> SSFKKILGLSSKSHKKSKKMGLPPPYDESSPMETQPSAPLSNDFFGMEDMDLYDKDSLRYEKFRFMLKMTVRSNKPFRSYDDVTAAVSQWDNSYIGMVGKRPFYKIIALIGSSHLQATPAVLADLNQPEYYATLTGRCFLPHRLGLIPPMFNVSETFRKPFNIGIYKGTLDFTFTVSDDESNEKVPHVWEYMNPKYQSQIQKEGLKFGLILSKKATGTWVLDQLSPFK

The rhabdovirus matrix (M) protein is small (∼20–25 kDa) but plays a number of roles during the replication cycle of the virus. The M protein is an important structural component of rhabdovirus virions, forming a layer between the glycoprotein- (G-) containing outer membrane and the nucleocapsid core composed of the virus nucleoprotein (N), polymerase (L), phosphoprotein (P) and RNA genome. In addition to its structural roles, M has been implicated in controlling the balance between transcription and replication of the viral genome, in promoting budding, and in modulating host-cell transcription, -translation and -apoptosis. To further investigate the role of the N terminus and hydrophobic surface-exposed loop and to investigate the structural conservation of M across Rhabdoviridae, we solved the structures of full-length M from VSV serotype New Jersey (VSVNJ) and from the lyssavirus Lagos bat virus (LBV).

The structure of VSVNJ M was solved by SeMet single-wavelength anomalous dispersion phasing and refined to 1.83 Å resolution with residuals R/Rfree = 0.157/0.179. VSVNJ M forms a globular domain with a central α helix sandwiched on one side by an extensive 5-stranded β sheet and on the other by two α helices and a smaller two-stranded β sheet that is very similar to the thermolysin-resistant core of M (Mth) from VSV serotype Indiana (VSVInd), with 0.9 Å root-mean-squared displacement (rmsd) over 156 Cα atoms. Residues 121–128, disordered in the VSVInd Mth structure, are observed in the structure of VSVNJ M with residues 121–124 forming a short stretch of α helix (α2.5). The N-terminal 57 residues of VSVNJ M do not form part of this globular domain. While residues 1–40 and 53–57 are not well ordered and could not be modeled in electron density, residues 41–52 are located in strong electron density bound in a deep hydrophobic pocket formed by the loops between sheet β1 and helix α1, the region between helices α2 and α2.5 (including sheet β2), and the stretch of 3–10 helix immediately preceding helix α3. F46 is central to the interaction: the side chain of F46 sits deep in the hydrophobic pocket lined by the side chains of residues Y81, V84, L116, Y131, Y197 and the backbone between residues 114 and 116. Overall, these interactions bury 1050 Å2 of surface area. The interaction of the globular domain with the N-terminal peptide of an adjacent molecule in the crystal gives rise to non-covalently linked linear polymers of VSVNJ M monomers. In VSVNJ M this loop has shifted toward the interacting N-terminal residues: the Cα atom of K196 moves 9.5 Å from its position in VSVInd Mth and residues 195–200 form a stretch of 3–10 helix. Our structure reveals that the Rae-1 binding site on VSV M partially overlaps with the N-terminal self-association motif.> GHMARSVRHIAIPAHRGLITDRNGEPLAVSTPVTTLWANPKELMTAKERWPQLAAALGQDTKLFADRIEQNAEREFIYLVRGLTPEQGEGVIALKVPGVYSIEEFRRFYPAGEVVAHAVGFTDVDDRGREGIELAFDEWLAGVPGKRQVLKDRRGRVIKDVQVTKNAKPGKTLALSIDLRLQYLAHRELRNALLENGAKAGSLVIMDVKTGEILAMTNQPTYNPNNRRNLQPAAMRNRAMIDVFEPGSTVKPFSMSAALASGRWKPSDIVDVYPGTLQIGRYTIRDVSRNSRQLDLTGILIKSSNVGISKIAFDIGAESIYSVMQQVGLGQDTGLGFPGERVGNLPNHRKWPKAETATLAYGYGLSVTAIQLAHAYAALANDGKSVPLSMTRVDRVPDGVQVISPEVASTVQGMLQQVVEAQGGVFRAQVPGYHAAG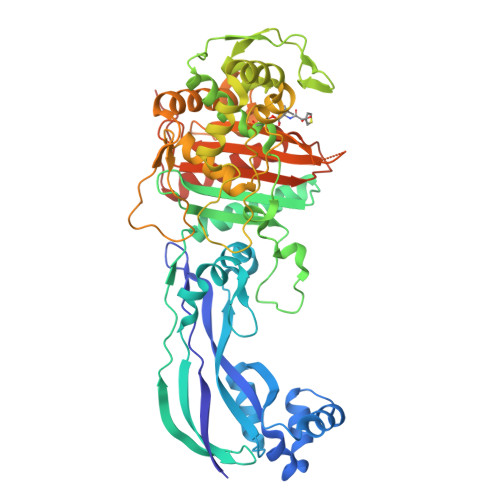KSGTARKVSVGTKGYRENAYRSLFAGFAPATDPRIAMVVVIDEPSKAGYFGGLVSAPVFSKVMAGALRLMNVPPDNLPTATEQQQVNAAPAKGGRG1-aminopropan-2-one | C3 H7 N O | 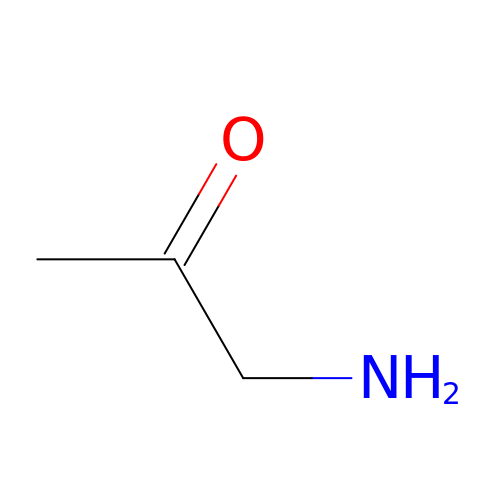BCDGQXUMWHRQCB-UHFFFAOYSA-N>[2x]GPHMRKIIIAGNWKMHKTQAEAQAFLQGFKPLIEDAAESREVVLCVPFTDLSGMSQQLHGGRVRLGAQNVHWEASGAYTGEISAAMLTEIGIHYVVIGHSERRQYFGETDETANLRVLAAQKAGLIPILCVGESKAQRDAGETEQVIVDQVKKGLVNVDQSNLVIAYEPIWAIGTGDTCAATEANRVIGLIREQLTNSQVTIQYGGSVNANNVDEIMAQPEIDGALVGGASLEPQSFARIVNFQP

Triosephosphate isomerase (TPI) interconverts glyceraldehyde-3-phosphate (G3P) and dihydroxyacetone phosphate (DHAP) near diffusion rate-limiting during glycolysis and the Calvin-Benson cycle. In most organisms, TPI is an obligated dimer that folds into a (β-α)8 barrel known as the TIM barrel. Thus, in land plants the ancestral cyanobacterial TPI originally present in chloroplasts was replaced by a duplicated version of the cytosolic TPI. Herein we found that Synechocystis TPI (SyTPI) is highly resistant to oxidative agents, suggesting that TPIs from prokaryotic photosynthetic organisms evolved to cope with ROS at the expense of redox regulation.

In order to have a structural understanding for the insensibility of SyTPI to H2O2 and thiol-conjugating agents, we growth protein crystals of SyTPI in complex with 2-phosphoglycolate (2-PG) that diffracted at a resolution of 1.6 Å. Resolution of the crystallographic data revealed that SyTPI assembles as a homodimer and that each monomer folds into a canonical (β-α)8 or TIM-barrel composed of eight α-helices and eight parallel β-strands. The active site of SyTPI shows that the catalytic residues Lys 11, His96, and Glu165 are poised in close contact with the inhibitor 2-PG. A superimposition of the crystal structure of SyTPI with TPIs crystalized in the absence of ligand (AtcTPI and AtpdTPI) illustrates that SyTPI exhibits a closed loop 6 conformation. SyTPI harbors a deletion of 7 amino acids in the loop that connects α-helix 6 with β-strand 7. In AtcTPI and AtpdTPI this region folds as a short α-helix, whereas this region in SyTPI folds as a loop that connects α-helix 6 and β-strand 7. SyTPI contains three cysteines per monomer. The thiol group of residue SyTPI-C127 is completely buried, whereas the thiol group of SyTPI-C176 contains the only accessible thiol group in this protein. A ribbon representation centered at residue SyTPI-C176, shows that this amino acid directly interacts with residues Y201 and S203 from the conserved loop 6 (phosphate-binding loop). An electrostatic map near residue SyTPI-C176 shows that this residue is surrounded by amino acids that have a negative electrostatic potential (D174, E212, E180) limiting the potential of this residue to react with GSSG or with H2O2.>[8x]MLTDNWKELAGKAQSTFQKSLKQAIELADFDEGLAKRYGALPSAIGANVEDFGSPAQFPLEEYLKALPKKVLDITEKDPVELLKDLKSRKVTCVEVLKAYTAASIVASKLTNCVQEFLPIEALQYAQKLDADYETKKHLPLYGLPFSIKEMIPFVGRSVTHGSLCYLDRIVDYNADIVNILIANGAYPFVRTTNPQSLMMLECVSFSHGRTVNAYNGMLTSGGSSGGEGALNGMRASPFGLGSDIGGSIRCPAAFNGIYGLRSTLGRIPTADYFSCNRGSESILSVTGPLSRSLDTVNLVMKTVIEAKPWLIDPTLVPLDWKRPENKKFRVGIYVSDHIVNPSPPINRALSMVTEKLKSLGNFEVVTFEPYKPEKVTEILGKLYFEDGARDFRATLQTGEPLLEQTRWAIEGAEDLDMHDQWYW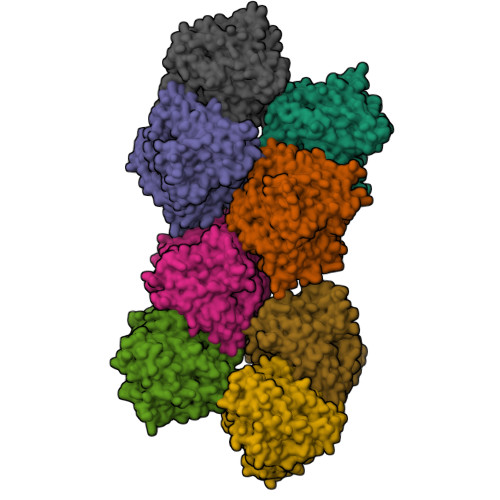NLQKQAYRKEFLKHWCSYTDNDGNVLDAVIAPVFPNVAAKHETTKYWTYTSQWNLLDYPVLAFPVTKVDESLDQPYKNYKPLNDLDKYFYEQYDSPSSFKNAPANLCLVGLRFTDEKLVEIANILRN>GPGHMPEYQAQGLAMYLQENGIDCPKCKFSYALARGGCMHFHCTQCRHQFCSGCYNAFYAKNKCPEPNCRVKKSLHGHHPRDCLFYLRDWTALRLQKLLQDNNVMFNTEPPAGARAVPGGGCRVIEQKEVPNGLRDEACGKETPAGYAGLCQAHYKEYLVSLINAHSLDPATLYEVEELE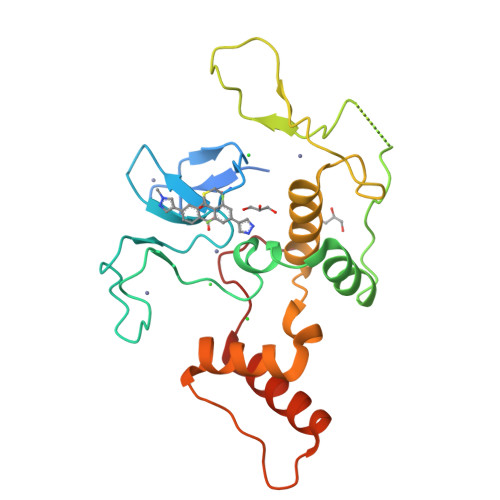TATERYLHVRPQPLAGEDPPAYQARLLQKLTEEVPLGQSIPRRRK[6x]(2S,5R,6S)-2-benzyl-5,6-bis(4-chlorophenyl)-4-methylmorpholin-3-one | C24 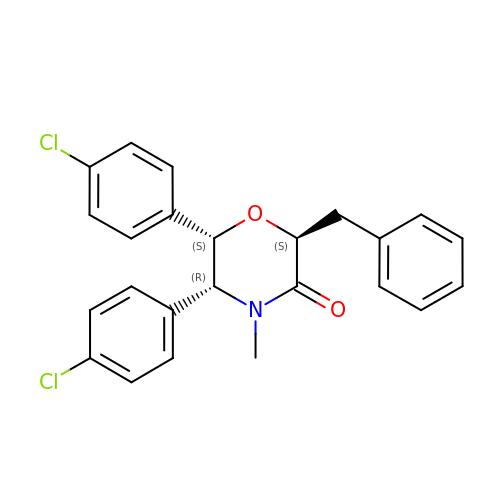H21 Cl2 N O2 | NFFXQTHZDQEVMP-ZRBLBEILSA-N>GMVRISIAGGNEIDPGSMGLTLFHEHLRLITEVVRWNWPHLYNEDEELKRAIDAVNAAKKYGVKTIIDLTVAGIGCDVRFNEKVAKATGVNIIMGTGFYTYTEIPFYFKNRGIDSLVDAFVHDITIGIQGTNTRAAFVKAVIDSSGLTKDVEMAIRAAAKAHIKTDVPIITHSFVGNKSSLDLIRIFKEEGVDLARTVIGHVGDTDDISFIEQILREGAFIGLDRFGLDIYLPLDKRVKTAIELIKRGWIDQLLLSHDYCPTIDWYPPEVVRSTVPDWTMTLIFEKVIPRMRSEGITEEQINRVLIDNPRRLFTGR[2x]

VmoLac (YP_004245953) is a recently identified enzyme that was isolated from the hyperthermophilic crenarchaeon Vulcanisaeta moutnovskia strain 768-2833. The phylogenetic tree that was built from this sequence alignment, indicates that VmoLac belongs to the clade of the PLLs-A. Kinetic characterization indicates that VmoLac is a proficient lactonase with promiscuous, poor esterase and phosphotriesterase activities. As expected, VmoLac is roughly globular and exhibits a (β/α)8 barrel topology that is similar to that of others PLLs such as SsoPox17, SisLac8, DrOPH3, GsP10 and GkL36.

The structure of VmoLac bound to its substrate 3-oxo-C10 AHL enabled us to identify the specific interactions of the enzyme with the bound lactone. Crystals of VmoLac were soaked with 3-oxo-C10 AHL, and the lactone sits in the hydrophobic channel of the active site. The omit density map cannot be confounded with that of the fatty acid, since the bound lactone is shorter, and the lactone ring is visible in the electronic density map. The lactone ring sits on the bi-metallic active site, while the carbonyl oxygen is bound to the β-Co (2.4 Å), and the esteric oxygen contacts the α-Co (2.4 Å). The carbonyl oxygen of the lactone ring also interacts with the Y98 O-H (2.3 Å) and the R224 guanidinium group (3.5 Å). The 1-oxo group weakly interacts with C259 (3.7 Å), and the long aliphatic chain sits in the hydrophobic channel that is formed by loop 8. The overall binding of the 3-oxo-C10 AHL is very similar to the previously observed binding of a lactone mimic, the inhibitor C10 homocysteine lactone in the SsoPox structure. A deeper comparison highlights the fact that the lactone ring is closer to the bi-metallic center in the VmoLac structure compared to the thiolactone ring in SsoPox. Moreover, the difference in the loop 8 conformation between both enzyme yield to a very different binding crevice, where very different residues are involved in the substrate binding, such as Y265VmoLac/T265SsoPox, V274VmoLac/A275SsoPox, T273VmoLac/L274SsoPox, and also V269VmoLac, V270VmoLac, A266SsoPox and Y270SsoPox. This different crevice results in the aliphatic chain binding outside loop 8 in VmoLac, whereas it binds inside loop 8 in SsoPox17. We surmise here that the hydrolysis mechanism of lactones by VmoLac is therefore close to those that have been previously proposed for SsoPox17.>VPRGSQNFLFGCELKADKKEYSFKVEDDENEHQLSLRTVSLGASAKDELHVVEAEGINYEGKTIKIA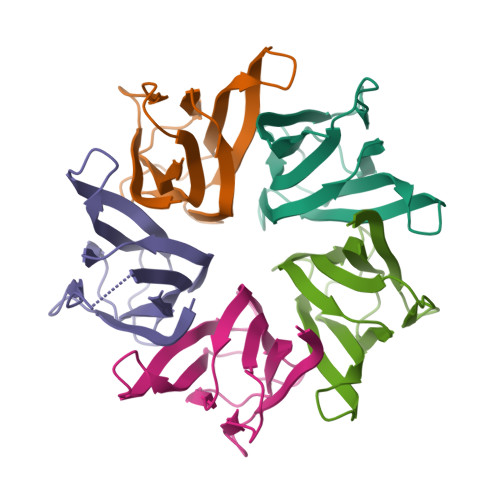LASLKPSVQPTVSLGGFEITPPVILRLKSGSGPVYVSGQHLVALEDL[10x]>[2x]MLLEAPVYKEIFGAVTIHEVQKVIKMDTETEEVPIYTISNIPREKIYDLLGKMAVIVPMKNEKLHLVDGVLKAIPHKCPIIIVSNSKREGPNRYKLEVDLIRHFYNLTHSKIIMIHQKDPGLAKAFKEVGYTDILDENGMIRSGKGEGMLVGLLLAKAIGAEYVGFVDADNYIPGAVNEYVKDYAAGFLMSESEYTMVR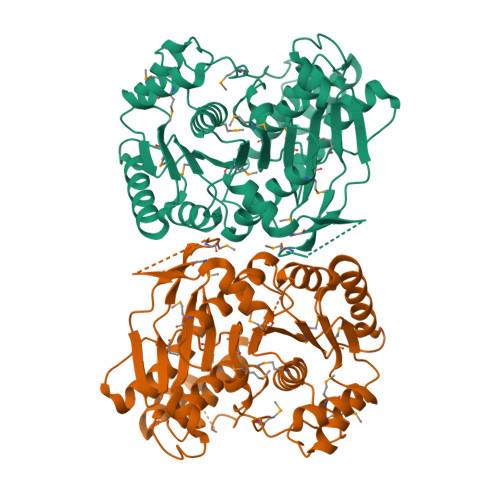LHWRHKPKVTKGTLYFKKWGRVSEITNHYLNLLVSEHTAFETTIMVTGNAGEHAMTMKLAEILPFSTGYSIEPYEIVYILERFGKWENVEEFKDVFDQGIEIFQIETLNPHFHEDKGKEHVKEMLLLSLATIYHSKLATDNLRKRILKDLRDHGILGENEEPPKPLVMRPIKEIPIKEWMDIVEGNSETLLRFEL> MWKTASDKGLGHLLRDVWSLLNEEERELLDKEIQPFPCKKASTVFSEGDIPNNLFYLYEGKIKILREGVYGRFHISRIVKPGQFFGMRPYFAEETCSSTAIAVENSKVLAIPVEAIEALLKGNTSFCRYFLKALAKELGYAERR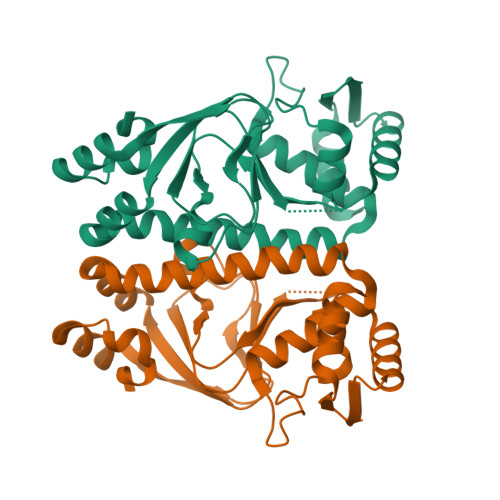TVTLTQKHVRGRLAETLLILKENFGFENDGATLSIYLSREELATLSNMTVSNAIRTLSTFVSERMLALDGKRIKIIDCDRLQKTARSG The ϕRSA1 bacteriophage has been isolated from Ralstonia solanacearum, a gram negative bacteria having a significant economic impact on many important crops. The ϕRSA1 capsid is composed solely of the polymerization of the major capsid protein, gp8, which exhibits the typical “Johnson” fold first characterized in E. coli bacteriophage HK97. As opposed to the latter, the ϕRSA1 mature capsid is not stabilized by covalent crosslinking between its subunits, nor by the addition of a decoration protein. Phage’s capsids are primarily composed of the major capsid protein (MCP), which assembles as hexamers and pentamers called the capsomers that ultimately form a closed icosahedral shell with the portal/connector complex located at one of the capsid’s vertices.

We solved the three-dimensional structure of the ϕRSA1 mature capsid to 3.9 Å resolution by cryo-electron microscopy. The capsid follows an icosahedral symmetry characterized by a triangulation number T = 7, dextro (d) in which the 11 out of the 12 vertices are made of pentamers (the last one is the portal connected to the tail) while the flatter facets are made of hexamers. Accordingly, there are seven unique quasi equivalent subunits of gp8 that composed the asymmetric unit of the ϕRSA1 capsid for a total of 415 subunits in the capsid. The core of the subunit is composed of the Axial (A) and Peripheral (P) domains to which the more flexible N-terminal (N) domain and Extended (E) loop are attached. Whereas the ϕRSA1’s capsid MCP core remains very similar (mean RMSD = 0.94 ± 0.16 Å) between the seven pairs of MCPs of the asymmetric unit, the N domain and the E loop can be displaced by as much as 12 and 20 Å, respectively, between the seven quasi equivalent subunits of the asymmetric unit in order to adapt to different local environments. In total, each MCP interacts with eight others: two are from the same capsomer, while the other six are spread across three different adjacent capsomers. The analysis of the various subunit–subunit interactions reveals that there are five main interfaces which can explain all the intra and inter capsomer’s interactions. The G-loop of ϕRSA1, which is longer than in most phages, acts as a sort of lock for the E-loop. Interestingly, ϕRSA1 doesn’t display either additional densities or any continuous density between the two subunits interacting at the 3-fold axis, which leads to the conclusion that ϕRSA1 uses none of the most common mechanisms to stabilize its capsid at the 3-fold. It follows that ϕRSA1 solely relies on interactions between its MCPs to get a strong enough assembly which can sustain the high pressure inside the capsid caused by the packaging of its genome.

>[7x]MRNDTRRLFAAYKAAIAKLNGVERVDEKFSVAPSVQQKLETKVQESSDFLKSINFYGVPEQEGEKIGLGVSGPVASTTDTTQQDRETSDISTMDGRRYRCEQTNSDTHITYQKLDAWAKFADFQTRIRDAIIKRQALDRIMIGFNGVSRAATSDRVANPMLQDVNKGWLQNLREQAPQRVMKEGKAAAGKITVGGAGADYGNLDALVYDITNHLVEPWYAEDPDLVVVCGRNLLSDKYFPLVNRDRDPVQQIAADLIISQKRIGNLPAIRVPYFPANGLLVTRLDNLSIYYQEGGRRRTILDNAKRDRIENYESSNDAYVIEDLACAAMAENIALAAAA>MIYTVTFNPSIDYVIFTNDFKIDGLNRATATYKFAGGKGINVSRVLKTLDVES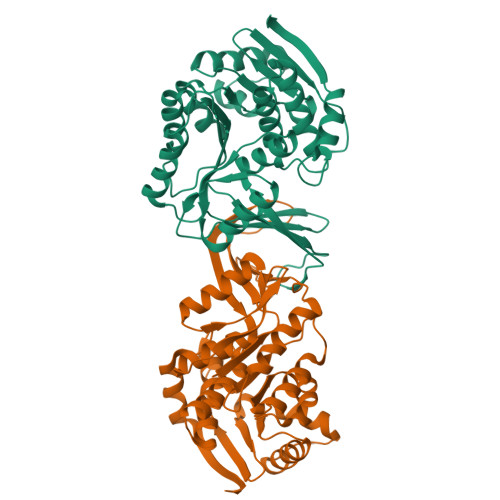TALGFAGGFPGKFIIDTLNNSAIQSNFIEVDEDTRINVKLKTGQETEINAPGPHITSTQFEQLLQQIKNTTSEDIVIVAGSVPSSIPSDAYAQIAQITAQTGAKLVVDAEKELAESVLPYHPLFIKPNKDELEVMFNTTVNSDADVIKYGRLLVDKGAQSVIVSLGGDGAIYIDKEISIKAVNPQGKVVNTVGSGDSTVAGMVAGIASGLSIEKAFQQAVACGTATAFDEDLATRDAIEKIKSQVTISVLDGE[2x]> GALERLPDGPRIHVPRKTALRPTVARQVFQPAFAPAVLSKFDPRTDADVDEVAFSKHTSNQETLPPVFRMVAREYANRVFALLGRDNGRLSVKQALDGLEGMDPMDKNTSPGLPYTTLGMRRTDVVDWETATLIPFAAERLEKMNNKDFSDIVYQTFLKDELRPIEKVQAAKTRIVDVPPFEHCILGRQLLGKFASKFQTQPGLELGSAIGCDPDVHWTAFGVAMQGFERVYDVDYSNFDSTHSVAMFRLLAEEFFSEENGFDPLVKDYLESLAISKHAYEEKRYLITGGLPSGCAATSVLNTIMNNIIIRAGLYLTYKNFEFDDVKVLSYGDDLLVATNYQLNFDRVRTSLAKTGYKITPANKTSTFPLESTLEDVVFLKRKFKKEGPLYRPVMNREALEAMLSYYRPGTLSEKLTSITMLAVHSGKQEYDRLFAPFREVGVIVPTFESVEYRWRSLFW

The genome is replicated via a negative-sense RNA intermediate by 3Dpol, the viral RNA-dependent RNA polymerase (RdRP). For this, 3Dpol uses the viral protein 3B, in this context usually termed VPg (viral protein genome-linked), as a primer. Crystal structures have been reported of 3Dpol of the enteroviruses CVB3, PV, EV71, HRV1B, HRV14, and HRV16, and of the aphthovirus FMDV. These enzymes adopt a classical right hand architecture, with fingers, palm and thumb subdomains providing the correct geometrical arrangement of substrate molecules and metal ions at the polymerase active site for catalysis. Given its critical role in genome replication, 3Dpol is regarded as an attractive target for antiviral drugs.

Interestingly, the three virus pools each contained a single missense mutation compared to wild-type (wt) virus. These mutations were located either at nucleotide 7115 (A7115G) or 7127 (A7127G) resulting in amino acid changes M300V and I304V in the viral RdRP, 3Dpol, respectively. Markedly higher inhibition constants were observed for the two resistant mutants (M300V, 26.9 μM; I304V, 10.3 μM) as compared to that for the wt enzyme (1.3 μM). The apo structures of the EMCV M300V and I304V polymerase mutants were obtained using the same crystallization conditions as for the wt enzyme, yielding two different types of crystals for the mutants. The M300V mutant crystallized in the space group I4122 form with one 3Dpol molecule in the asymmetric unit (a.u.) and diffracted to 2.2 Å resolution. Structural comparisons showed that the mutant polymerases were almost identical to the wt enzyme. The main differences were concentrated in helix α10, which contains the mutated residues, and in the preceding loop B. The side chains of residues 300 and 304 participate in a large hydrophobic cluster linking α10 with helices α2 (Y75), α6 (F194, A195, F199), α7 (I210) and α8 (L241, F255 and F256), included in the inner fingers. The substitutions of the methionine and isoleucine side chains by the shorter valine in the mutants imply a weakening of these hydrophobic interactions. This could result in an increased flexibility of α10, including the disruption of the last helical turn, and of the B-loop, which appears to have a key role in GPC-N114 binding in EMCV 3Dpol. In addition, the substitution with valine may disrupt the interaction of residue 300 with the compound. The structures of the EMCV 3Dpol M300V and I304V mutants suggest that these mutations increase the flexibility of this loop, thereby affecting the binding site of GPC-N114 and probably losing a direct interaction with the shorter V300 side chain whilst retaining the ability to interact with the template-primer.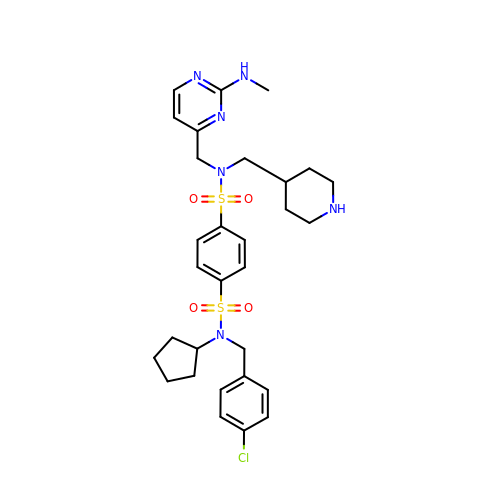~{N}1-[(4-chlorophenyl)methyl]-~{N}1-cyclopentyl-~{N}4-[[2-(methylamino)pyrimidin-4-yl]methyl]-~{N}4-(piperidin-4-ylmethyl)benzene-1,4-disulfonamide | C30 H39 Cl N6 O4 S2 | FWBBCSKXUXMTJY-UHFFFAOYSA-N>[6x]GSHMETYNVELVRKDGQSLGIRIVGYVGTSHTGEASGIYVKSIIPGSAAYHNGHIQV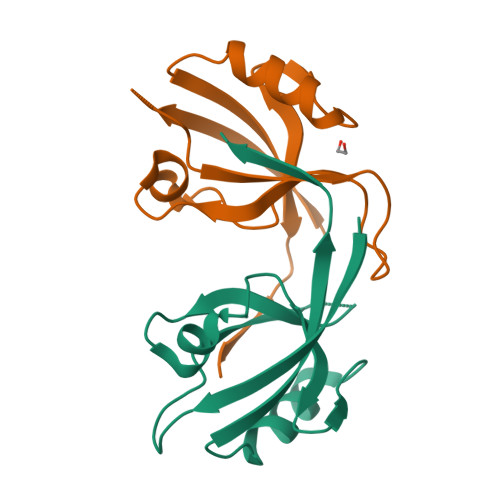NDKIVAVDGVNIQGFANHDVVEVLRNAGQVVHLTLVRRGGGWFLDI> APAVA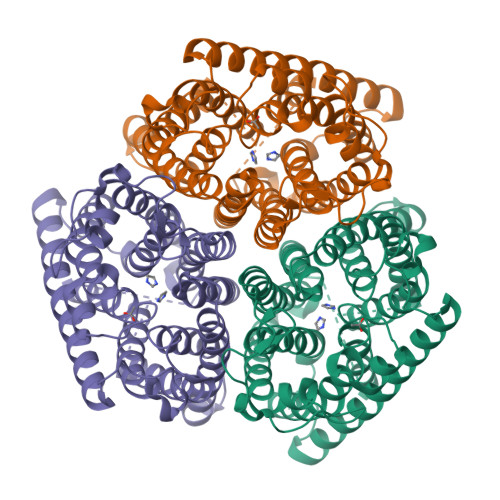DKADNAFMMICTALVLFMTIPGIALFYGGLIRGKNVLSMLTQVTVTFALVCILWVVYGYSLAFGEGNNFFGNINWLMLKNIELTAVMGSIYQYIHVAFQGSFACITVGLIVGALAERIRFSAVLIFVVVWLTLSYIPIAHMVWGGGLLASHGALDFAGGTVVAINAAIAGLVGAYLIGKRVGFGKEAFKPHNLPMVFTGTAILYIGWFGFNAGSAGTANEIAALAFVNTVVATAAAILGWIFGEWALRGKPSLLGACSGAIAGLVGVTPACGYIGVGGALIIGVVAGLAGLWGVTMLKRLLRVDDPCDVFGVHGVCGIVGCIMTGIFAASSLGGVGFAEGVTMGHQLLVQLESIAITIVWSGVVAFIGYKLADLTVGLRVPEEQEREGLDVNSHGENAYNADQAQQPAQADLEHHHHHH>[3x]SNAMVQRVTIAPQGPEFSRFVMGYWRLMDWNMSARQLVSFIEEHLDLGVTTVDHADIYGGYQCEAAFGEALTLAPHLREKLQIVTKCGIATTARAENKLGHYITDRRHIILSAEQSLKNLATDYLD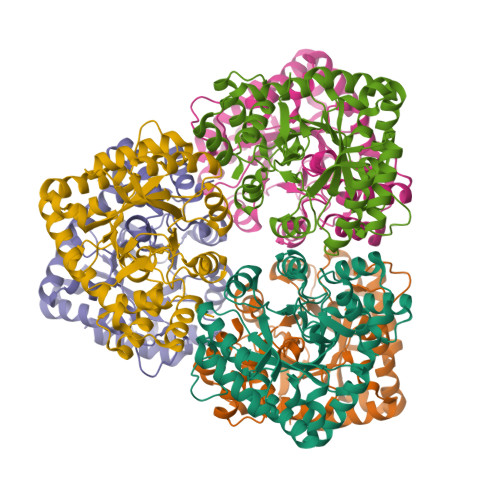MLLIHRPDPLMDADDVAEAFQHLHQSGKVRHFGVSNFTPAQFTLLQSRLPFTLATNQVEISPVHQPLLLDGTLDQLQQLRIRPMAWSCLGGGRLFNDEAYQPLRQELSVIAQELNASSIEQVVYAWILRLPSQPLPIIGSGKIERVRAALEAETLSLTRQQWFRIRKAALGYDVP>GSHMVTIVRI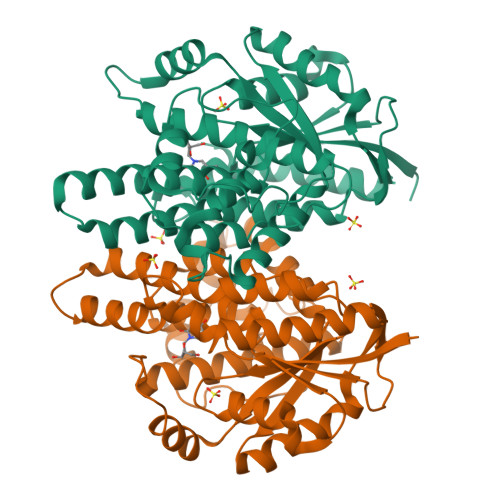YLDGVYGIGKSTTGRVMASAASGGSPTLYFPEPMAYWRTLFETDVISGIYDTQNRKQQGNLAVDDAALITAHYQSRFTTPYLILHDHTCTLFGGNSLQRGTQPDLTLVFDRHPVASTVCFPAARYLLGDMSMCALMAMVATLPREPQGGNIVVTTLNVEEHIRRLRTRARIGEQIDITLIATLRNVYFMLVNTCHFLRSGRVWRDGWGELPTSCGAYKHRATQMDAFQERVSPELGDTLFALFKTQELLDDRGVILEVHAWALDALMLKLRNLNVFSADLSGTPRQCAAVVESLLPLMSSTLSDFDSASALERAARTFNAEMGV[2x]> MAHAGRTGYDNREIVMKYIHYKLSQRGYEWDAGDDVEE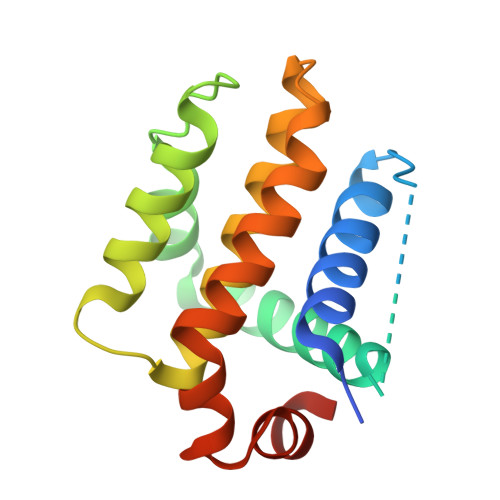NRTEAPEGTESEVVHLTLRQAVDDFSRRYRRDFAEMSSQLHLTPFTARGRFATVVEELFRDGVNWGRIVAFFEFGGVMCVESVNREMSPLVDNIALWMTEYLNRHLHTWIQDNGGWDAFVELYGPSMR>AMSLNIITVTLNMEKYNFLGISIVGQSNERGDGGIYIGSIMKGGAVAADGRIEPGDMLLQVNEINFENMSNDDAVRVLREIVHK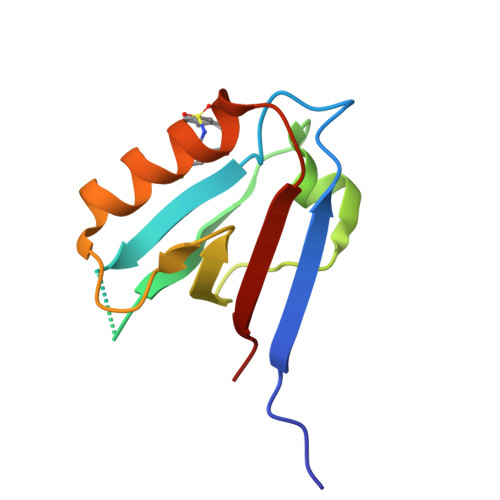PGPITLTVAKS[2x]(3R,5S,9R)-1-[(2R,3S,4R,5R)-5-(6-amino-9H-purin-9-yl)-4-hydroxy-3-(phosphonooxy)tetrahydrofuran-2-yl]-3,5,9-trihydroxy-8,8-dimethyl-10,14-dioxo-2,4,6-trioxa-11,15-diaza-3,5-diphosphaheptadecane-17-sulfinic acid 3,5-dioxide (non-preferred name) | C21 H36 N7 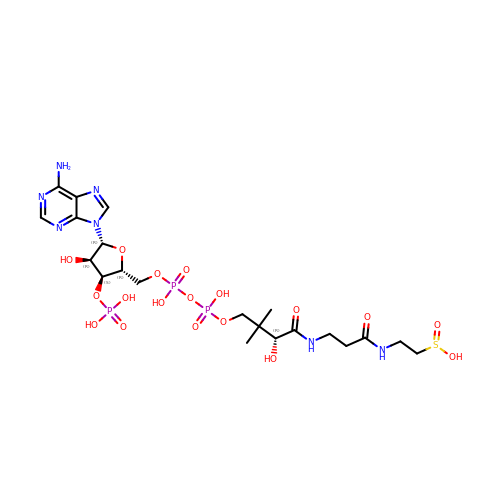O18 P3 S | HHNOQZRCHLIIMA-IBOSZNHHSA-N One example is the sperm-specific SLC9C1 that belongs to the SLC9 superfamily of cation/proton antiporters, known as Na+/H+ exchangers (NHEs), which are essential for the regulation of intracellular pH, sodium homeostasis and cell volume. The transport domain (TD) is accompanied by a voltage-sensing domain (VSD) and a cyclic-nucleotide binding domain (CNBD), which are regulatory units usually found in voltage-gated cyclic-nucleotide-modulated ion channels, also referred to as CNBD ion channels. In a recent patch-clamp fluorimetry study, the functional integrity of the domains was confirmed for SLC9C1 from the sea urchin Strongylocentrotus purpuratus, termed SpSLC9C1, identifying it as a Na+/H+ exchanger that is activated strictly by hyperpolarization and modulated by cyclic nucleotides (cNMPs). Specifically, SpSLC9C1 adapted to mediate cellular alkalization in sperm only in response to chemoattractant-induced hyperpolarization.

In contrast, all membrane-embedded domains were better resolved when reconstituted into nanodiscs, yielding a map at 3.2 Å that was used for subsequent model building. SpSLC9C1 adopts an inward-facing conformation, similar to the majority of eukaryotic NHE structures, with the residues of the binding site accessible from the cytoplasm forming a negatively charged cavity. The voltage-sensing helix S4 is in the inactive upward position, as no activating hyperpolarizing conditions can be established in detergent or nanodiscs. All positively charged residues reside within the membrane and R1 (R803), which is homologous to R368 in Shaker Kv and is supposed to cross the entire membrane electric field upon activation, is still high above the gating charge transfer centre (GCTC). Prominent examples are the clear densities corresponding to two lipids embedded in the cavity found at the extracellular half of the dimer interface of the TD. Further, they form a cytoplasmic dimer interface and interprotomer interactions, with helices CH1 and CH2 of one protomer wedged between the helix pair CH8’–CH9’ and the CNBD of the adjacent protomer. Further, we could identify a network of salt bridges between CH4 and the core domain of the TD (E606–H157, R609–D155, K224–E616), which might contribute to locking the transporter in the inward conformation. Another interesting position is K939 on CH9, which is coordinated by E300, and backbone carbonyl groups located in the dimer domain. Under non-activating conditions, the TD is locked in an inward-facing state through interactions with coupling helices (state 1).

>MSKKRVVKLRELVPAVAALAVAVLIQSATGSSGGSGHTPTTQATHADDHDLTTHNGTEEHDDGHDDGHDDLHAHAPKVIVFISGSCLFGAISRSLFKKLPIPYTVVLLILGAILGVVASNVPLVEEHTRDVAHMDPHVLLQIFLPVLIFESAFAMDVHTFMRSFSQVCILALFGLVVASVLTAVLAMNLFNYNWNFSEAMMFGAIMSATDPVAVVALLKDLGASKQLGTIIEGESLLNDGCAIVIFNVFMKMVFFPQLTSTVGQNVLYFLQVAVAGPLWGYAVAKVTVFFLSHIFNDALVEITITLAATYLTYYIGDIWLEVSGVLAVVVLGLIVNAEKTSISPEVEVFLHRFWEMLAYLANTLIFMMVGVVVTQKALVAVDKMDWFYLIILYLAITIIRGMVISLFSPILSRIGYGLTWRNAVIMTWGGLRGAVGLALALVVENLAGNDVIGSKFLFHTAGIVVLTLVINATTIQTLLRILGMSDISIPKRLAMAGAVRRIHEGQNRTLNMLKSDRFLADADWDIATAACEISDPYSALSDDENAPADELTLGERKSVCPGCKAMVPNEPSPREFADMMEEARLRMLKAEKISYWKQFEHGMLAREALRLLVQHAEVAADEKDQFILVDDLKKSWQIKGIYPWLKRKLEDLISEKKIAAIPMPKYKLGKLMYKICHHMAFEVTINIAIVLNIVPIIMEFVVQDKMASVSTMAAPGSTVSSEPSSLQKIEDALRISNYVFFVIYAIEAIVKILGLGRHYIVSHWNKFDAFILVVALVDIIIAETLLKGSITINLSSIKVVKLFRLLRGLRMLRLTKALIPKLILVVNGKINNQLSLGYDVGKGYIIGEEEVGKIIDRMVDNKKILRELKHISETGRLQVVKELGLLQREHPGIAVSVKTRQAIRTILNHSRETIHELQGAGLLDEMEAHKLELTVEIKMKRLMNAPSSIPPPPPENLLKNVSWLAGDMKLIDFIKARASLLHFDYGEVIVREGDESDGLFLIVSGLVKLYGKSAFLDHDNPPVTAGSEENEVFEDYLTVGNVIGEMGVLTKKPRNATVTCETTVQVYFITAEDMNIAIDTFTLYPSLEYRLWRVVAIRIATPLIMEQMAFQGWTQEKVKLHLERGYLVDLAESHFQFNIDATLEDVILINGTAYNAHTREEIRSPCLISRTVHKLTFQYTATEEPRLFVVRNAEYNGPILDGRLDVDSKRSLISITEISSNMCLKHAAELRQKNSKVMLSRKSSGAAAKEEEDCIPNTSDVEQAAGVSPSVPTKTTPKPKSFLPSLGLSMSKERVNGEAVEESPVKTKQGEETPETEEGAAPRVNVALEVLFQ[2x]(3,4,5,7-TETRAHYDROXY-HEPT-1-ENYL)-PHOSPHONIC 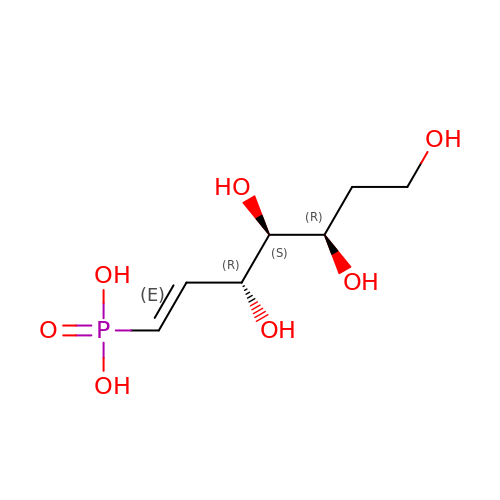ACID | C7 H15 O7 P | CZQSGBWQBMZTMQ-AEVYZNAZSA-N> GTHHHHHHHHGSQNETEPIVLEGKCLVVCDSNPTSDPTGTALGISVRSGSAKVAFSAIRSTNHEPSEMSNRTMIIYFDQVLVNIGNNFDSERSTFIAPRKGIYSFNFHVVKVYNRQTIQVSLMLN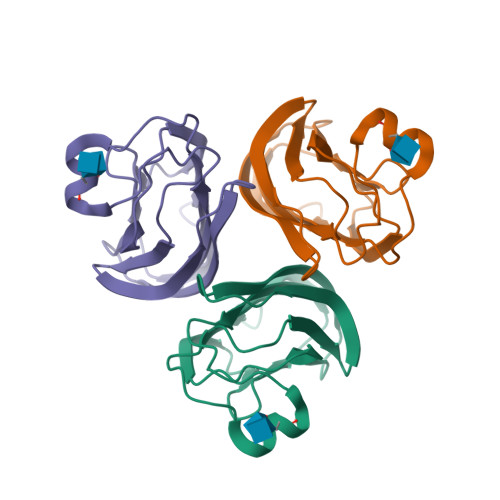GWPVISAFAGDQDVTREAASNGVLIQMEKGDRAYLKLERGNLMGGWKYSTFSGFLVFPL> GSRPADPEIVEGLPIPLAVAGHHQPAPFYLTADMFGGLPVQLAGGELSTLVGKPVAAPHTHPVDELYLLVSPNKGGARIEVQLDGRRHELLSPAVMRIPAGSEHCFL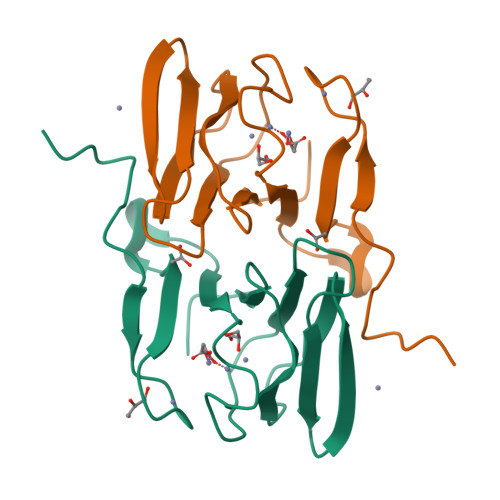TLEAEVGSYCFGILLGDRL ethyl 1-(cyclohexylmethyl)-5-pyridin-4-yl-indole-2-carboxylate | C23 H26 N2 O2 | 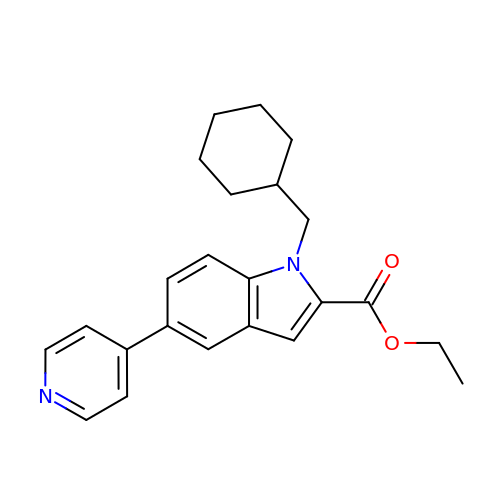NNPMKHYWTMMCKN-UHFFFAOYSA-N>ALALYTPLPTPTGWTTMGDVAVGDELLGADGKPTRVVAATDVMLGRPCYEVEFSDGTVIVADAAHQWPTSGGIRTSAQLRSGADRIVVAGSAGGYAEQRSATGLLVPVVQIESARRVASVPVRCVEVDNPAHLYLAGRGMVPTHN[2x]

Protein splicing is catalyzed by intervening protein sequences termed inteins. The protein-splicing reaction involves the self-removal of the intein and concomitant joining of the two flanking sequences (exteins). All splicing domains found among inteins have the same structural architecture named HINT (Hedgehog/INTein) which relates to the C-terminal domain of the Hedgehog protein (Hh–C or hog domain). Instead of the N-terminal serine or cysteine missing among class 3 inteins, class 3 inteins contain an additional nucleophilic cysteine residue in block F.

We determined the high-resolution crystal structures of two variants of the class 3 MchDnaB1 intein (MchDnaB1_HN and MchDnaB1_HAA). We found that the most striking feature of the crystal structures of the MchDnaB1 intein is the active site, closely resembling the catalytic triad of serine/cysteine proteases. The WCT motif found in the class 3 intein participates in forming the catalytic triad, in which Cys124, His65, and Thr143 could serve as nucleophilic, basic, and acidic functional groups, respectively. Importantly, we could observe clear electron density near the side-chains of Cys124, His65, and the backbone of Val125 for both crystal structures of the MchDnaDB1_HN and MchDnaB1_HAA inteins (modeled as oxyanion waters in Figure 2a and Supplemental Figure S2). However, the crystal structures of both MchDnaB1 intein variants (HN and HAA at the C-terminus) lacked electron densities for the N-extein sequences. This observation is presumably due to self-cleavage at the N-terminus during sample preparation and/or crystallization (N-cleavage). We observed electron density for both the gauche+ and trans-like conformations of Cys124 in the crystal structure of MchDnaB1_HN, although the side-chain conformation of Cys124 in the trans-like conformation is less evident in the second molecule (chain B) in the asymmetric unit. Upon removal of the N-extein in the simulation, the population largely shifted towards the ideal gauche+ conformation with χ1 = ~300° (−60°), with more frequent rotation between gauche+ and trans-like conformations. This observation might suggest that both crystal structures represent the post-splicing or post-cleavage status as expected from the primary structure of the variants. The intein will reach the ground state (gauche+ conformation of Cys124), represented by the crystal structure of MchDnaB1_HN.>HHHHHHFNLPPGNYKKPKLLYCSNGGHFLRIDPNGTVDGTRDRSDQHIQLQLSAESVGEVYIKSTETGQYLAMDTDGLLYGSQTPNEECLFLERLEENHYNTYISKKHAEKNWFVGLKKNGSCKRGPRTHYGQKAILFLPLPVSSD[2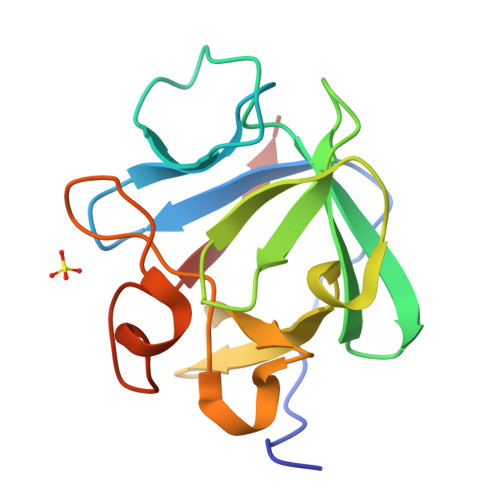x]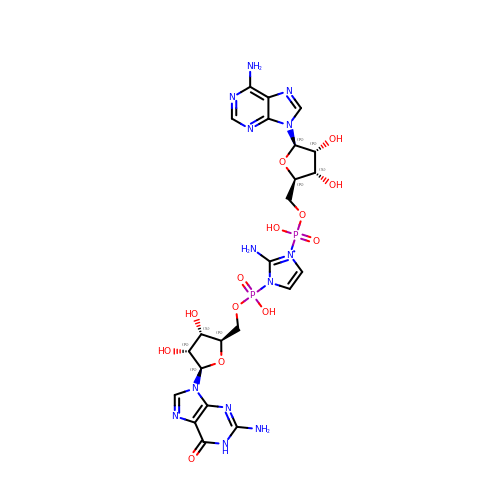[(2~{R},3~{S},4~{R},5~{R})-5-(6-aminopurin-9-yl)-3,4-bis(oxidanyl)oxolan-2-yl]methoxy-[2-azanyl-3-[[(2~{R},3~{S},4~{R},5~{R})-5-(2-azanyl-6-oxidanylidene-1~{H}-purin-9-yl)-3,4-bis(oxidanyl)oxolan-2-yl]methoxy-oxidanyl-phosphoryl]imidazol-1-yl]phosphinic acid | C23 H30 N13 O13 P2 | UTMQQHPBLGAUQK-NAGRZYTCSA-N HuR/ELAVL1 is an RNA-binding protein involved in differentiation and stress response that acts primarily by stabilizing messenger RNA (mRNA) targets. HuR specifically recognizes adenine and uridine-rich elements (ARE) and uridine-rich sequences in 3′ untranslated regions (3′UTRs) of mRNAs. Hu/ELAV proteins share a common protein architecture with two consecutive RRMs, separated from the third RRM (RRM3) by a less conserved, flexible hinge region of variable length. Here, we report crystal structures of HuR RRM3 free and bound to U- and AU-rich RNAs.

We initially selected two 6-mer RNA substrates: a sequence comprising the AUUUA pentamer derived from an ARE in TNF-α 3′UTR, (AU6tnf – UAUUUA), and a poly-U RNA that can be found in class III ARE elements without AUUUA repeats (U6 – UUUUUU). Both RNAs were bound by RRM3, with a Kd of 156 μM and 19 μM, respectively. It thus seems plausible that the lower Kd of RRM3 binding to U6 results from both avidity due to binding in multiple registers and preference for U-rich over AUUUA motifs. We observed a substantial increase in RRM solubility after RNA binding and were thus able to use untagged RRM3 incubated with selected RNA ligands for structural studies of the complex. This allowed us to perform a comprehensive and comparative analysis of RRM3 interaction with three distinct RNA ligands: AUUUA motif-containing (AU6tnf), a U-rich motif with sparsely distributed adenosine residues (AU15) and a poly-U motif (U6). While in the structure of RRM3 with U6 and AU15, a uridine is recognized, in the case of AU6tnf RNA, an adenosine is bound in this pocket. On the 3′ end of the RNA, nucleotides in positions 5 and 6 are closer to the RRM3 β2β3 loop in case of the U6 ligand than when AU15 or AU6tnf are bound. Interestingly, the β2β3 loop that is in close proximity to the 3′ end of the RNA in the crystal structure of the RRM3–U6 RNA complex appears to be most significantly affected by U6 titration. To summarize, the core of the RNA interactions with RRM3 is formed by three binding pockets with canonical aromatic residues from RNP2 and RNP1 (Phe247, Tyr249, Phe289) that recognize a U–U–U/A RNA sequence motif. The affected area correlates best with the dimeric interface found between chains A and B in the structures of RNA-bound RRM3 suggesting this is the dimerization interface in solution.

>MGWCIFIYNLGQDADEGILWQMFGPFGAVTNVKVIRDFNTNKCKGFGFVTMTNYEEAAMAIASLNGYRLGDKILQVSFKTNKSHK[3x]> TKNKD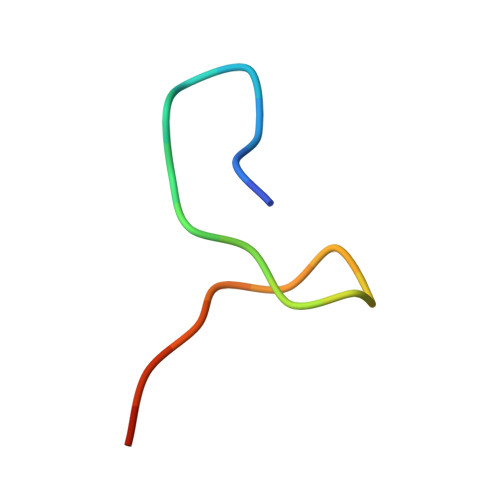GVLVDEFGLPQIPAS Tweety homologs (TTYHs) are conserved transmembrane proteins present in all eukaryotes including three members (TTYH1, TTYH2, and TTYH3) in humans. TTYHs have been reported to form Ca2+- and cell volume-regulated anion channels structurally distinct from any characterized protein family with potential roles in cell adhesion, migration, and developmental signaling. Each protomer consists of five transmembrane helices (TM1–5) and an extracellular domain (ED) which extends 75 Å from the membrane surface between an extracellular N-terminus and intracellular C-terminus. We conclude TTYHs are not pore forming subunits of anion channels and their function may involve Ca2+-dependent changes in quaternary structure, interactions with hydrophobic molecules near the extracellular membrane surface, and/or association with additional protein partners.

To test this, we purified and reconstituted TTYH2 into lipid nanodiscs without Ca2+ and in the presence of EGTA to maintain low free Ca2+ concentrations for structure determination. The Ca2+-free TTYH2 cryo-EM data did reveal a change in oligomeric state, but surprisingly we identified two different conformations in approximately equal proportions: the expected monomeric TTYH2 (to 4.0 Å resolution) and an unexpected head-to-head homodimer (a “trans-dimer” to 3.9 Å resolution) in which TTYH2 protomers embedded in separate nanodiscs associate via a buried surface at the distal end of each ED. The trans-dimer therefore bridges two opposing membranes over a ~130 Å extracellular space. The trans-dimeric interface is smaller than the cis-dimeric interface, burying 908 Å2 compared to 1556 Å2 and is largely polar with eight intersubunit hydrogen bonds (between residues D166-Q316, D166-T320, Q169-T321, and Q325-Q325), π-π stacking interactions (between F173-F173), and nonpolar interactions (between I324-L329). The trans- and cis-dimeric interfaces are partially overlapping with residues Q316, R317, T320, and T321 each contributing to both TTYH2 cis-dimer and trans-dimer interactions. As a consequence of this partial overlap in interfaces, cis-dimerization and trans-dimerization are expected to be mutually exclusive. In mouse TTYH2, the RGD motif (R164, G165, D166) is positioned at the distal tip of the ED within the short linker between helices EDH1 and EDH2. Indeed, the RGD motif forms part of the trans-dimerization interface in TTYH2. In contrast, it is exposed in TTYH2 cis-dimers and monomers with ~250 Å2 of solvent accessible area presented to solution by each RGD. This difference suggests that if RGD or RGD-like motifs in TTYHs do interact with integrins, the interaction could be regulated by extracellular Ca2+ levels: cis-dimers favored in the presence of Ca2+ would display RGDs available for interaction, while trans-dimerization in low Ca2+ conditions would disfavor integrin interaction by sequestration of the RGD surface.

>[2x]PAARVEYIAPWWVVWLHSVPHLGLRLQRVDSTFSPGDETYQESLLFLGVLAAIGLGLNLIFLTVYLVCTCCCRRDHTVQTKQQESCCVTWTAVVAGLLCCAAVGVGFYGNSETNDGMHQLIYSLDNANHTFSGMDELVSANTQRMKVDLEQHLARLSEIIAARGDYIQTLKFMQQMAGNVVSQLSGLPVWREVTTQLTKLSHQTAYVEYYRWLSYLLLFILDLVICLVTCLGLARRSKCLLASMLCCGILTLILSWASLAADAAAAVGTSDFCMAPDIYILNNTGSQINSEVTRYYLHCSQSLISPFQQSLTTFQRSLTTMQIQVGGLLQFAVPLFPTAEKDLLGIQLLLNNSEISLHQLTAMLDCRGLHKDYLDALTGICYDGIEGLLFLGLFSLLAALAFSTLTCAGPRAWKYFINRDRDYDDIDDDDPFNPQARRIAAHNPTRGQLHSFCSYSSGLGSQCSLQPPSQTISNAPVSEYMNQAILFGGNPRYENVPLIGRGSPPPTYSPSMRPTYMSVADEHLRHYEFPSSNSLEVLFQ>[2x]MSELFSERIPPQSIEAEQAVLGAVFLDPTALTLASERLIPEDFYRAAHQKIFHAMLRVADKGEPVDLVTVTAELAALEQLEEVGGVSYLSELADSVPTAANVEYYARIVEEKSLLRRLIRTATSIAQDGYTREDEIDVLLDEAERKIMEVSQRKHSGAFKN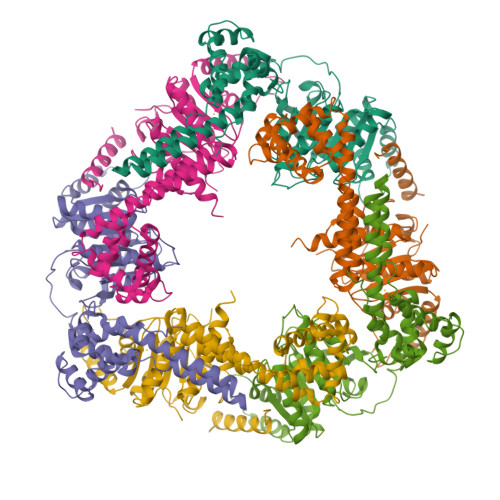IKDVLVQTYDNIEMLHNRNGDITGIPTGFTELDRMTSGFQRSDLIIVAARPSVGKTAFALNIAQNVATKTNENVAIFSLEMSAQQLVMRMLCAEGNINAQNLRTGKLTPEDWGKLTMAMGSLSNAGIYIDDTPSIRVSDIRAKCRRLKQESGLGMVVIDYLQLIQGSGRNRENRQQEVSEISRSLKALARELEVPVIALSQLSRSVEQRQDKRPMMSDLRESGSIEQDADIVAFLYRDDYYNKDSENKNIIEIIIAKQRNGPVGTVQLAFIKEYNKFVNLERRFDEAQIPPGA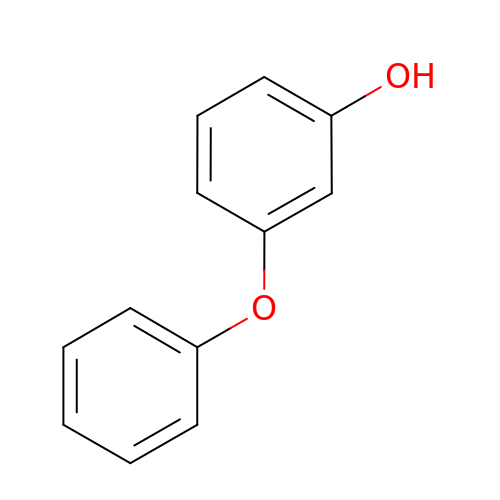3-phenoxyphenol | C12 H10 O2 | HBUCPZGYBSEEHF-UHFFFAOYSA-N>[2x]MFEQRVNSDVLTVSTVNSQDQVTQKPLRDSVKQALKNYFAQLNGQDVNDLY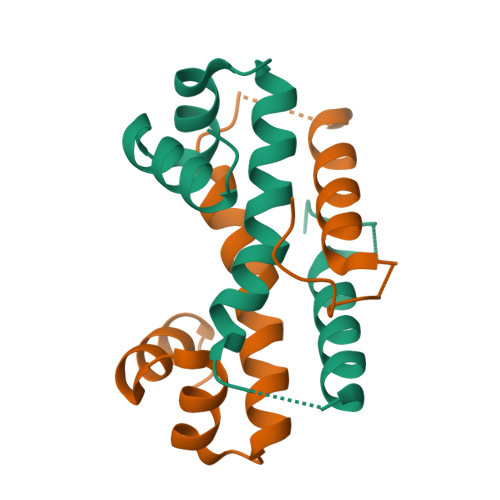ELVLAEVEQPLLDMVMAYTRGNQTRAALMMGINRGTLRKKLKKYGMN> SKFLDRFRYFKQKGETFADGHGQLLNTNRDWEDGYRQRWQHDKIVRSTHGVNCTGSCSWKIYVKNGLVTWETQQTDYPRTRPDLPNHEPRGCPRGASYSWYLYSANRLKYPMMRKRLMKMWREAKALHSDPVEAWASIIEDADKAKSFKQARGRGGFVRSSWQEVNELIAASNVYTIKNYGPDRVAGFSPIPAMSMVSYASGARYLSLIGGTCLSFYDWYCDLPPASPQTWGEQTDVPESADWYNSSYIIAWGSNVPQTRTPDAHFFTEVRYKGTKTVAVTPDYAEIAKLCDLWLAPKQGTDAAMALAMGHVMLREFHLDNPSQYFTDYVRRYTDMPMLVMLEERDGYYAAGRMLRAADLVDALGQENNPEWKTVAFNTNGEMVAPNGSIGFRWGEKGKWNLEQRDGKTGEETELQLSLLGSQDEIAEVGFPYFGGDGTEHFNKVELENVLLHKLPVKRLQLADGSTALVTTVYDLTLANYGLERGLNDVNCATSYDDVKAYTPAWAEQITGVSRSQIIRIAREFA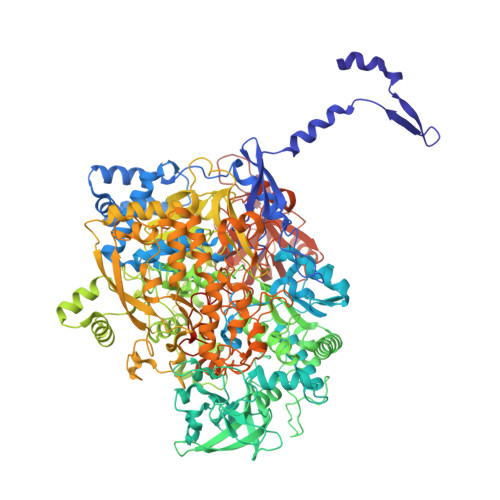DNADKTHGRSMIIVGAGLNHWYHLDMNYRGLINMLIFCGCVGQSGGGWAHYVGQEKLRPQTGWQPLAFALDWQRPARHMNSTSYFYNHSSQWRYETVTAEELLSPMADKSRYTGHLIDFNVRAERMGWLPSAPQLGTNPLTIAGEAEKAGMNPVDYTVKSLKEGSIRFAAEQPENGKNHPRNLFIWRSNLLGSSGKGHEFMLKYLLGTEHGIQGKDLGQQGGVKPEEVDWQDNGLEGKLDLVVTLDFRLSSTCLYSDIILPTATWYEKDDMNTSDMHPFIHPLSAAVDPAWEAKSDWEIYKAIAKKFSEVCVGHLGKETDIVTLPIQHDSAAELAQPLDVKDWKKGECDLIPGKTAPHIMVVERDYPATYERFTSIGPLMEKIGNGGKGIAWNTQSEMDLLRKLNYTKAEGPAKGQPMLNTAIDAAEMILTLAPETNGQVAVKAWAALSEFTGRDHTHLALNKEDEKIRFRDIQAQPRKIISSPTWSGLEDEHVSYNAGYTNVHELIPWRTLSGRQQLYQDHQWMRDFGESLLVYRPPIDTRSVKEVIGQKSNGNQEKALNFLTPHQKWGIHSTYSDNLLMLTLGRGGPVVWLSEADAKDLGIADNDWIEVFNSNGALTARAVVSQRVPAGMTMMYHAQERIVNLPGSEITQQRGGIHNSVTRITPKPTHMIGGYAHLAYGFNYYGTVGSNRDEFVVVRKMKNIDWLDGEGNDQVQESVK> MFEARLVQGSILKKVLEALKDLINEACWDISSSGVNLQSMDSSHVSLVQLTLRSEGFDTYRCDRNLAMGVNLTSMSKILKCAGNEDIITLRAEDNADTLALVFEAPNQEKVSDYEMKLMDLDVEQLGIPEQEYSCVVKMPSGEFARICRDLSHIGDAVVISCAKDGVKFSASGELGNGNIKLSQTSNVDKEEEAVTIEMNEPVQLTFALRYLNFFTKATPLS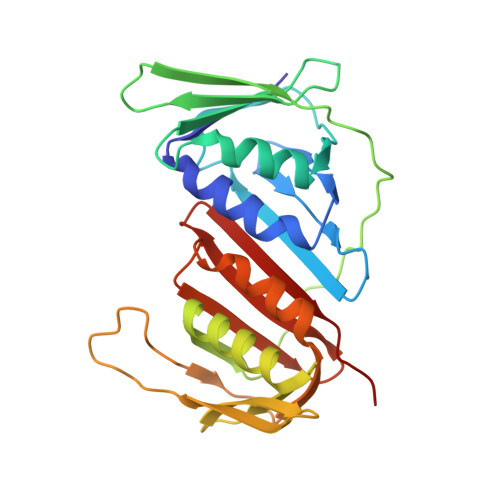STVTLSMSADVPLVVEYKIADMGHLKYYLAPKIE> GNTLVVLHKSGLL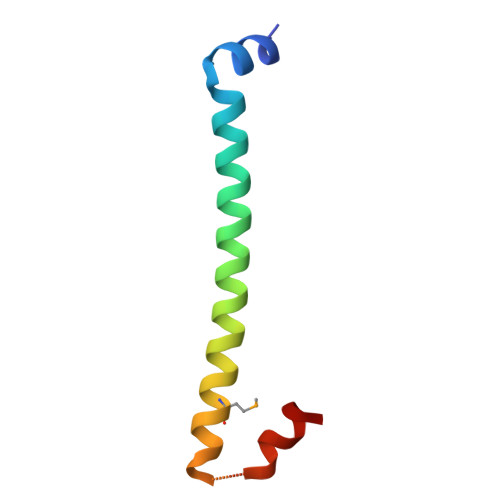EITLKTKELIRQNQATQAELDQLKEQTQMFIEATKSRAPQAWAKLQASLTS> MKTPSQPRAIYYIVAIQIWEYFSFYGMRALLILYLTHQLGFDDNHAISLFSAYASLVYVTPILGGWLADRLLGNRTAVIAGALLMTLGHVVLGIDTNSTFSLYLALAIIICGYGLFKSNISCLLGELYDENDHRRDGGFSLLYAAGNIGSIAAPIACGLAAQWYGWHVGFALAGGGMFIGLLIFLSGHRHFQSTRSMDKKALTSVKFALPVWSWLVVMLCLAPVFFTLLLENDWSGYLLAIVCLIAAQIIARMMIKFPEHRRALWQIVLLMFVGTLFWVLAQQGGSTISLFIDRFVNRQAFNIEVPTALFQSVNAIAVMLAGVVLAWLASPESRGNSTLRVWLKFAFGLLLMACGFMLLAFDARHAAADGQASMG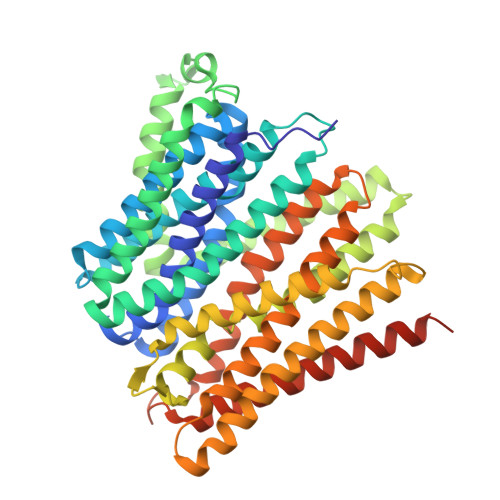VMISGLALMGFAELFIDPVAIAQITRLKMSGVLTGIYMLATGAVANWLAGVVAQQTTESQISGMAIAAYQRFFSQMGEWTLACVAIIVVLAFATRFLFSTPTNMIQESND>SNAFLDYGLSEADPDVHAIINKEKDRQFRSLELIASENFTSKAVMEAVGSCLTNKYSEGLPGKRYYGGNEHIDELEILCQQRALAAFHLDGDKWGVNVQPLSGSPANFAVYTAILKPHDRIMGLDLPHGGHLSHGFMTAKRRVSGTSIYFESMPYRLDESTGVIDYDMLEKTAALFRPKLIIAGASAYPRDIDYARFRKIADSVGAFLMMDMAHVSGLIAASVLADPFEFVDIVTTTTHKSLRGPRGGMIFFKKDAVHGVDLESAINNAVFPGLQGGPHNHTIGGLAVCLKYAQSPDFKNYQNQVVANCRALANRLVEHEYKLVSGGSDNHLVLVDLRPSGIDGARVEKILDMASITLNKNSVPGDKSALVPGGIRIGSPAMTTRGLGEKEFELIADLIHEGVRISLEAKSLVSGTKVQDFLNFVLAPEFPLGDKVSNLRRKVEALATQYPIPGV[8x]

SHMTs are α-class pyridoxal 5′-phosphate (PLP)-dependent enzymes which transfer hydroxymethyl of Ser to – typically polyglutamylated (polyGlu) – tetrahydrofolate (H4PteGlun), producing Gly and 5,10-CH2-H4PteGlun. Here we report crystal structures of a chloroplastic SHMT enzyme from the model legume plant, Medicago truncatula (Mt), which similarly to At has seven SHMT isoforms. MtSHMT3 is a member of the α-class of PLP enzymes, and its overall fold is typical for this family. A subunit of MtSHMT3 can be subdivided into three regions: N-terminal arm, large domain, and small domain, consistently with other SHMTs.

Soaking with Ser the MtSHMT3 crystal that grew in the presence of PEG and 150 mM ammonium acetate allowed to capture three snapshots along the course of reaction, killing the metaphorical three birds (intermediates) with one stone (crystal). The three different stages, within the asymmetric unit containing two tetramers are: PLP-Ser external aldimine (chains A and D), PLP-Gly external aldimine (chains B and F), and PLP internal aldimine with free Gly (chains E and H). PLP was bound at a partial occupancy or absent altogether in the chains G and C, respectively. Importantly, the reaction proceeded in the crystal despite H4PteGlun was not present in the crystallization milieu. The presence of Ser leads to the formation of Ser-PLP external aldimine, which changes the conformation of PLP moiety. However, creation of the covalent bond between PLP and Ser forces the rotation of the plane of the PLP ring ∼20° outwards from Nζ of K318. The side-chain of H292 is actually flipped to interact with the carboxyl group of the Ser moiety, salt-bridged in turn to R454, and H-bonded to Oγ of S114 and Oη of Y144∗. The complex with PLP-Ser external aldimine shows its unique conformation, with the PLP-Ser γ-hydroxyl group hydrogen-bonded to Y144∗ and synperiplanar to the PLP-Ser carboxyl C atom. This lineup, whereby the hydroxyl of Y144∗ also interacts with the PLP-Ser carboxyl, suggests Y144∗ as a potential base in the H4PteGlun-independent retroaldol cleavage. Y143∗ is shown to adopt a conformation ready to stack H4PteGlun in the states wherein the cosubstrate is needed in the active site (PLP-Ser and PLP-Gly external aldimines).> GEIQWVKPNKETGRLSINGPTRTKLEPSVFHDVFEGNKEPAVLHSKDPRLEVDFEQALFSKYVGNTLYEPDEYIKEAALHYANQLKQLEINTSQMSMEEACYGTENLEAIDLHTSAGYPYSALGIKKRDILDPTTRDVSKMKFYMDKYGLDLPYSTYVKDELRSIDKIKKGKSRLIEASSLNDSVY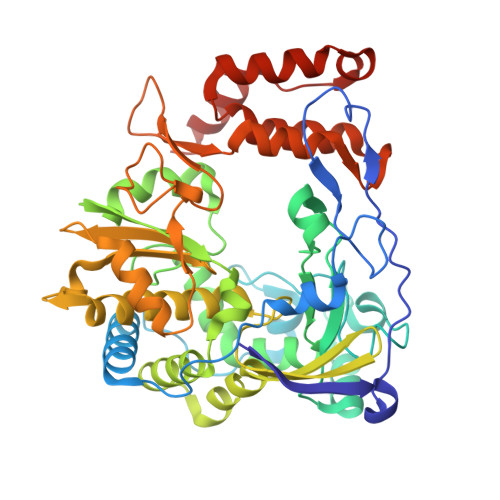LRMAFGHLYETFHANPGTITGSAVGCNPDTFWSKLPILLPGSLFAFDYSGYDASLSPVWFRALELVLREIGYSEEAISLIEGINHTHHVYRNKTYCVLGGMPSGCSGTSIFNSMINNIIIRALLIKTFKGIDLDELNMVAYGDDVLASYPFPIDCLELAKTGKEYGLTMTPADKSPCFNEVNWDNATFLKRGFLPDEQFPFLIHPTMPMREIHESIRWTKDARNTQDHVRSLCLLAWHNGKQEYEKFVSTIRSVPVGRALAIPNYENLRRNWLELF>MAPVLGYWKIRGLAQPIRLLLEYVGHSYEEHSYGRCDGEKWQNDKHNLGLELPNLPYYKDGNFSLTQSLAILRYIADKHNMIGNTPVERAKISMIEGGLVDLRAGVSRIAYQETFEQLKVPYLQQLPSTLRMWSQFLGNNSYLHGSTPTHLDFMFYEALDVIRYLDPTSVEAFPNLMQFIHRIEALPNIKAFMESDRFIKWPLNGWSAYF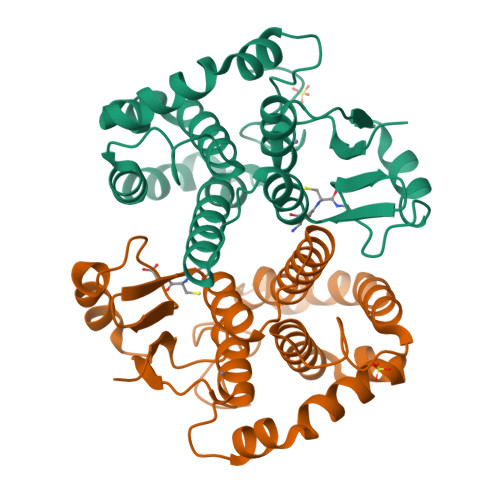GGGDAPPK[3x]>MILKPENEKKLIIDVLKKFGVPEEDAKITADVFVDADLKGFTSHGIGRFPQYITALKLGNINPKPDIKIVKESPATAVIDGDLGLGQVVGKKAMELAIKKAKNVG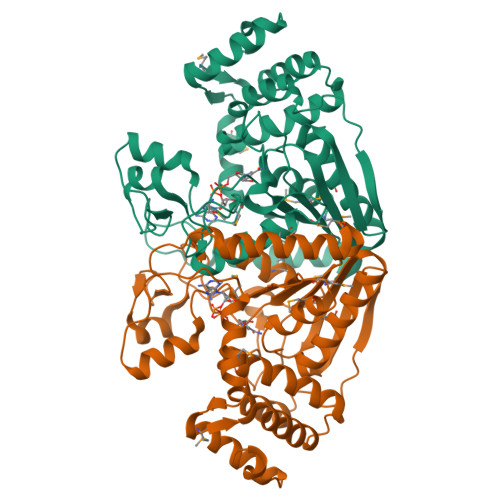VGVVATRNANHFGIAGYYSELAMNQDMIGITITNTEPAMAPFGGKEKILGTNPIAIAFKGNKYKFSLDMATASIARGKILEALRKKIKIPEGCAVDKDGKPTTDPAKALEGCILPFGGPKGYGLALAIEMLSAIGGAEVGTKVKGTANPEERCTKGDLFIAINPEFFMGKEEFKRKVDELLDEIKNSEPAEGFEILIPGEIEERNKMKRKDGFEIDKNLYNQLKEICNELGLNIEDYIE[8x]> EDPQGDAAQKTDTSHHDQDHPTFNKITPNLAEFAFSLYRQLAHQSNSTNILFSPVSIAAAFAMLSLGAKGDTHDEILEGLNFNLTEIPEAQIHEGFQELLHTLNQPDSQLQLTTGNGLFLSEGLKLVDKFLEDVKKLYHSEAFTVNFGDTEEAKKQINDYVEKGTQGKIVDLVKELDRDTVFALVNYIFFKGKWERPFEVKDTEEEDFHVDQVTTVKVPMMKRLGMFNIQHCKKLSSWVLLMKYLGNATAIFFLPDEGKLQHLENELTHDIITKFLENEDRRSA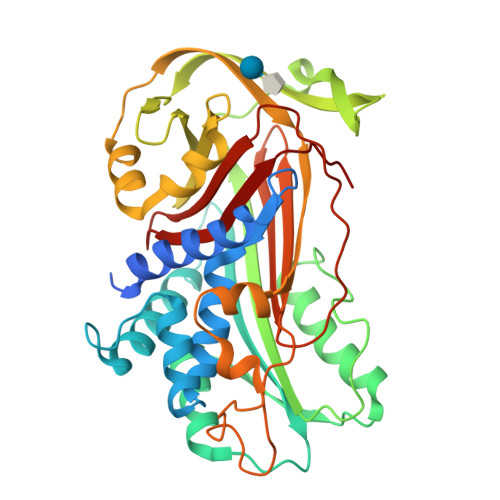SLHLPKLSITGTYDLKSVLGQLGITKVFSNGADLSGVTEEAPLKLSKAVHKAVLTIDEKGTEAAGAMFLEAIPMSIPPEAKFNKPFVFLIIDQNTKAPLFMGRVVNPTQK> MASMTGGQQMGRDEAGITGTWYNQLGSTFIVTAGADGALTGTYESAAGKAESRYVLTGRYDSAPATDGSGTALGWTVAWKNNYRNAHSATTWSGQYVGGAEARINTQWLLTA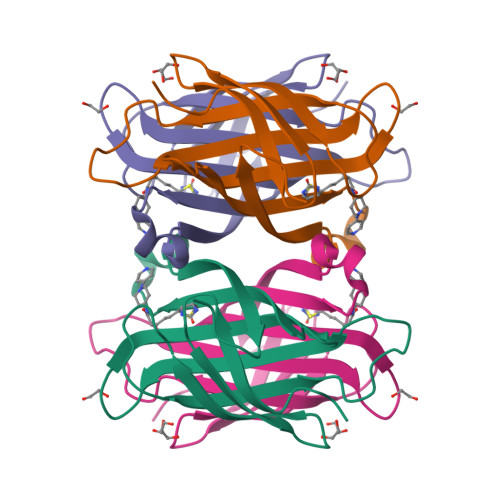GQTEANGWASTLVGHDTFTKVKPSAASIDAAKKAGVNNGNPLDAVQQ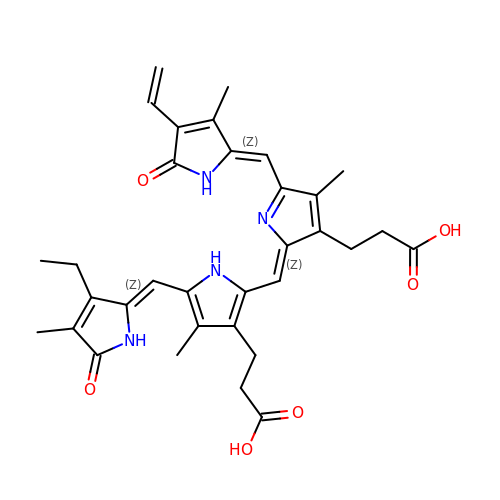3-[2-[(~{Z})-[5-[(4-ethenyl-3-methyl-5-oxidanylidene-pyrrol-2-ylidene)methyl]-3-(3-hydroxy-3-oxopropyl)-4-methyl-pyrrol-2-ylidene]methyl]-5-[(~{Z})-(3-ethyl-4-methyl-5-oxidanylidene-pyrrol-2-ylidene)methyl]-4-methyl-1~{H}-pyrrol-3-yl]propanoic acid | C33 H36 N4 O6 | OFLCQIQWTPZPJY-IRCLPSFSSA-N9-chloro-2-({5-[3-(dimethylamino)propyl]-2-methylpyridin-3-yl}amino)-5,7-dihydro-6H-pyrimido[5,4-d][1]benzazepine-6-thione 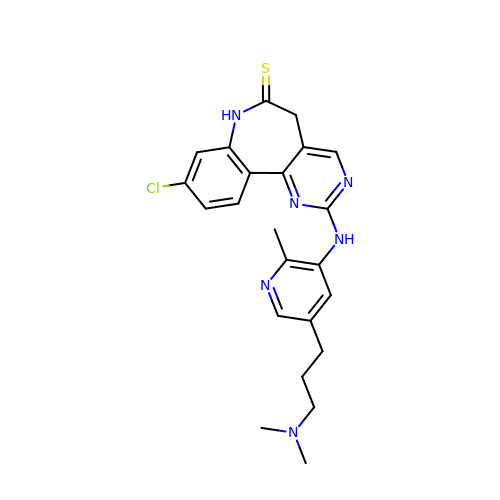| C23 H25 Cl N6 S | MYVQSDVXBZNNLF-UHFFFAOYSA-N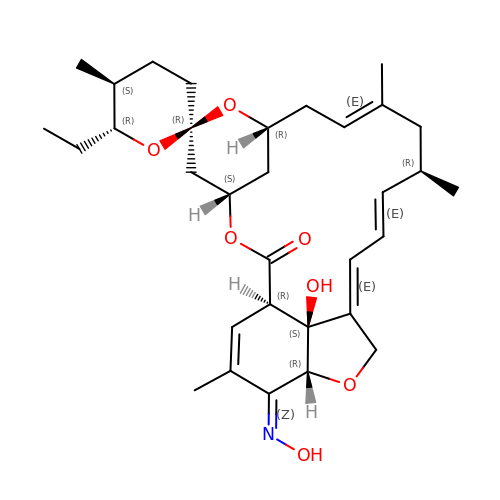milbemycin oxime | C32 H45 N O7 | YCAZFHUABUMOIM-JUBNYKKYSA-N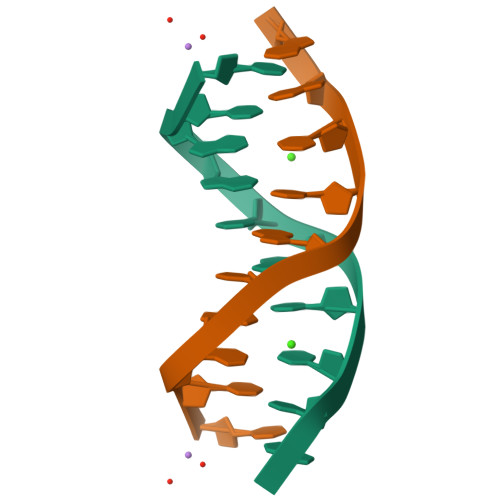> CCAACITTGG> QPNVDMGFEAAVAKKVVVPITFMVPNRPSGLTQSALLVTGRTFLINEHTWSNPSWTSFTIRGEVHTRDEPFQTVHFTHHGIPTDLMMVRLGPGNSFPNNLDKFGLDQMPARNSRVVGVSSSYGNFFFSGNFLGFVDSITSEQGTYARLFRYRVTTYKGWCGSALVCEAGGVRRIIGLHSAGAAGIGAGTYISKLGLIKALKHLGEPLATMQ

Seneca virus A (SVA) is an emerging novel picornavirus that has recently been identified as the causative agent of many cases of porcine vesicular diseases in multiple countries. The full-length SVA genome is approximately 7.3 kb in length and contains a single open reading frame (ORF) encoding a single polyprotein that undergoes proteolytic processing and cleavage by the viral 3C protease (3Cpro) into four structural proteins (VP4-VP2-VP3-VP1) and eight non-structural proteins (L-2A-2B-2C-3A-3B-3C-3D). SVA 3Cpro is composed of two topologically equivalent antiparallel six-stranded β-barrel domains (A1-F1 and A2-F2). Three closely positioned residues (His48, Asp84 and Cys160) within the proteolytic active site of SVA 3Cpro comprise the canonical catalytic triad.

In this work, we first report the crystal structure of wild-type SVA 3Cpro, which indicates that SVA 3Cpro adopts a chymotrypsin-like fold and possesses the Cys-His-Asp catalytic triad conserved in most serine proteases. Judging from the electron density of Cys160, the sulfhydryl group appears to have an alternate conformation (with an angle of ~120°orientation). During the refinement of the SVA 3Cpro structure, we observed a portion of extra electron density located in the cleft mainly composed of E1’-F1 loop and α3. The region is composed of dominantly positive residues, including His75, His78, His79, Arg147, Lys198 and His202, which neighbor the proteolytic site. Considering the rough shape of this the non-protein electron density and the complementary charges, we considered this as a phospholipid-like ligand. Based on the lipid-binding assay and lipidomics data, the CL 74:6 molecule (with a molecular composition of C83H150O17P2) was assigned to the identified electron density in SVA 3Cpro. The CL molecule, especially its two phosphate groups, was well defined in the electron density map after refinement. Interestingly, the C-terminus containing the natural autocatalytic processing site (GEPLATMQG) from Molecule II, inserts into the proteolytic active site of Molecule I. Therefore, despite a crystallography artefact formed by the two contacting molecules, the SVA 3Cpro-substrate complex likely captures the physiological peptide cleavage process of SVA 3Cpro. In our SVA 3Cpro–substrate complex structure, the main chain carbonyl carbon of the substrate Gln211 was 3.1 and 3.7 Å from each γ-sulfur atom (Sγ) in two alternative sulfhydryl groups of the Cys160 nucleophile. These distances imply that it would be difficult for Cys160 to covalently bind to Gln211 through a thioester linkage.(2~{R})-2-[[2-methyl-3-oxidanyl-5-(phosphonooxymethyl)pyridin-4-yl]methylamino]-3-oxidanyl-propanoic acid | C11 H17 N2 O8 P | 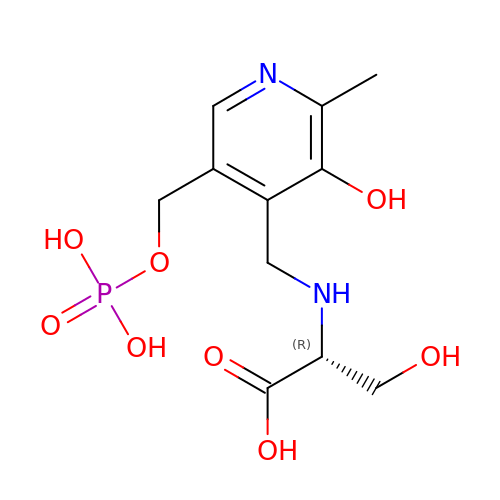ODVKKQWXKRZJLG-SECBINFHSA-N>MSNLKDFSQPGSGQESNFGVDFVIHYKVPAAERDEAEAGFVQLIRALTTVGLATEVRHGENESLLVFVKVASPDLFAKQVYRARLGDWLHGVRVSAPHNDIAQALQDEPVVEAERLRLIYLMITKPHNEGGAGVTPTNAKWKHVESIFPLHSHSFNKEWIKKWSSKYTLEQTDIDNIRDKFGESVAFYFAFLRSYFRFLVIPSAFGFGAWLLLGQFSYLYALLCGLWSVVFFEYWKKQEVDLAVQWGVRGVSSIQQSRPEFEWEHEAEDPITGEPVKVYPPMKRVKTQLLQIPFALACVVALGALIVTCNSLEVFINEVYSGPGKQYLGFLPTIFLVIGTPTISGVLMGAAEKLNAMENYATVDAHDAALIQKQFVLNFMTSYMALFFTAFVYIPFGHILHPFLNFWRATAQTLTFSEKELPTREFQINPARISNQMFYFTVTAQIVNFATEVVVPYIKQQAFQKAKQLKSGSKVQEDHEEEAEFLQRVREECTLEEYDVSGDYREMVMQFGYVAMFSVAWPLAACCFLVNNWVELRSDALKIAISSRRPIPWRTDSIGPWLTALSFLSWLGSITSSAIVYLCSNSKNGTQGEASPLKAWGLLLSILFAEHFYLVVQLAVRFVLSKLDSPGLQKERKERFQTKKRLLQENLGQDAAEEAAAPGIEHSEKITREALEEEARQASIRGHGTPEEMFWQRQR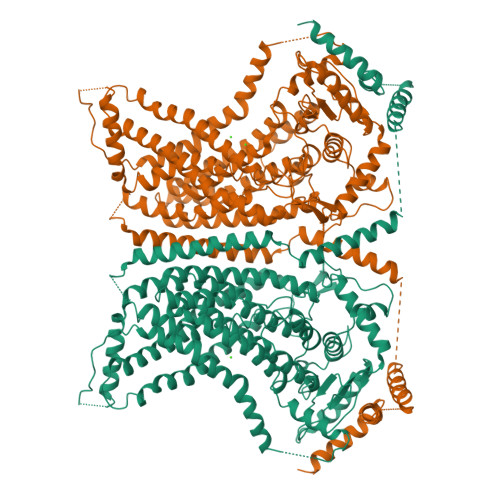GMQETIEIGRRMIEQQLAAGKNGKKSAPAVPSEKAS[2x]> GPNPQTEEVSIKEIAITHHVKEGHEKADPSQFELLKVLGQGSFGKVFLVKKISGSDA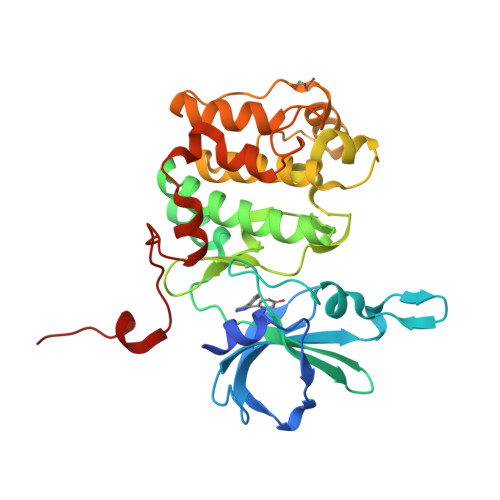RQLYAMKVLKKATLKVRDRVRTKMERDILVEVNHPFIVKLHYAFQTEGKLYLILDFLRGGDLFTRLSKEVMFTEEDVKFYLAELALALDHLHSLGIIYRDLKPENILLDEEGHIKLTDFGLSKESIDHEKKAYSFCGTVEYMAPEVVNRRGHTQSADWWSFGVLMFEMLTGTLPFQGKDRKETMTMILKAKLGMPQFLSPEAQSLLRMLFKRNPANRLGAGPDGVEEIKRHSFFSTIDWNKLYRREIHPPFKPATGRPEDTFYFDP>[2x]AVGPVTDIHIVNKDIAPDGFSRPSVLAGGTFPGPLITGQKGDNFKLNVVDD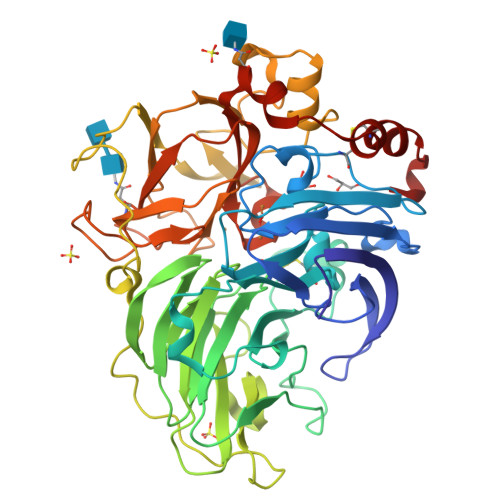LTDASMLKSTSIHWHGFFQKGTNWADGPAFVNQCPISTGNSFLYNFQVPDQAGTYWYHSHLSTQYCDGLRGAFVVYDPTDPHKALYDVDDESTVITLADWYHTLARQIVGVAIADTTLINGLGRNTNGPADAALAVINVEAGKRYRLRLVSISCDPNYVFSIDNHDFNIIEVDGVNSKPLNVDSIQIFAGQRYSAVLNANQPVGNYWVRANPNLGTTGFTGGINSAILRYKGAPVAEPTTTQTTSTKPLQEPNLRPLVSMPVPGSATPGGVDVVHNLILGFSAGKFTINGAAFTPPSVPVLLQILSGTTNAQDLLPSGSVITLPIGKTIELTLAAGVLGGPHPFHLHGHNFHVVRSAGQTTPNYVDPIVRDVVNTGGTGDNVTIRFTTDNPGPWFLHCHIDWHLEAGFAVVFAEGVNQTNAANPTPADWNNLCNIYNALADGDK Bilin 618 (single linked) | C33 H36 N4 O6 | 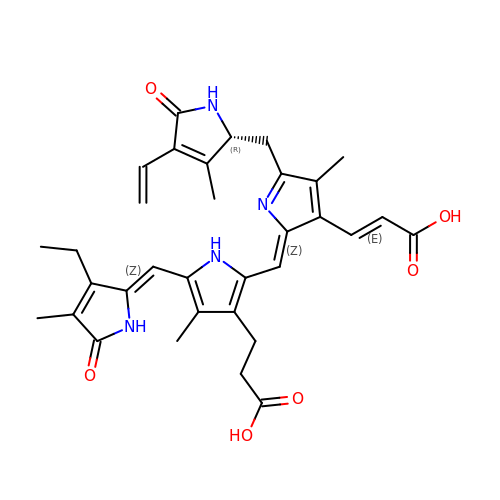DWOKJMXOEBXRPB-ZHKKBVGESA-N> MLKQVEIFTDGSCLGNPGPGGYGAI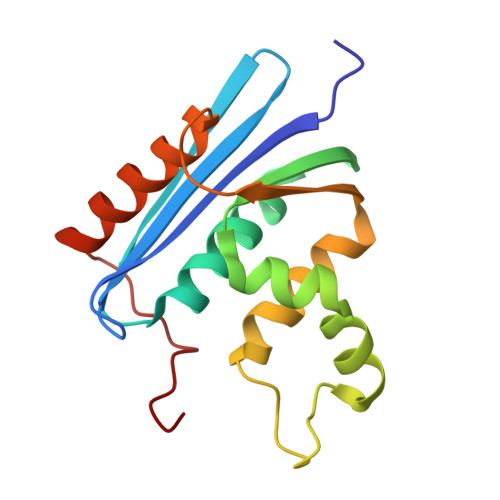LRYRGREKTFSAGYTRTTNNRMELMAAIVALEALKEHCEVILSTDSQYVRQAITQGWIHNWKKRGWKTADKKPVKNVDLWQRLDAALGQHQIKWEWVKGHAGHPENERCDELARAAAMNPTLEDTGYQVEV>GSMSKWTYFGPDGENSWSKKYPSCGGLLQSPIDLHSDILQYDASLTPLEFQGYNLSANKQFLLTNNGHSVKLNLPSDMHIQGLQSRYSATQLHLHWGNPNDPHGSEHTVSGQHFAAELHIVHYNSDLYPDASTASNKSEGLAVLAVLIEMGSFNPSYDKIFSHLQHVKYKGQEAFVPGFNIEELLPERTAEYYRYRGSLTTPPCNPTVLWTVFRNPVQISQEQLLALETALYCTHMDDPSPREMINNFRQVQKFDERLVYTSFSQ[4x]

The role of carbonic anhydrase isozyme IX (CAIX) in tumor cell survival, proliferation, migration, pH regulation, and cell-signaling pathways made this enzyme a promising therapeutic target in oncology. , Tumor cells primarily express two membrane-associated carbonic anhydrases, CAIX and CAXII. These isozymes belong to a family of zinc metalloenzymes that catalyze the reversible hydration of CO2 to form HCO3 – and H+. Although the active site is characterized by conserved amino acids between 12 isozymes, the amino acids further away from the zinc ion provide some variability. Crystal structures of CAIX and CAXII with five compounds by using soaking or cocrystallization were determined to confirm the binding mode of the ligands and reveal insights that govern enhanced affinity.

Four ligands in complexes with CAXII are of similar structures, contain a cyclooctylamine group at the 3-position and (3-hydroxypropyl)­sulfonyl tail at the 4-position, but vary in substituents at the 5-position: compound 9 has a (4-hydroxybutyl)­amino moiety, compound 10 - piperidinyl, compound 13 - methoxy, and compound 14 - ethoxy. The introduction of methoxy (compound 13) and ethoxy (compound 14) groups at the 5-position of fluorinated benzenesulfonamide 5c resulted in the most strongly binding compounds for CAIX, with the K d,obs reaching 4.5 pM at pH 7.0. Interestingly, cancer-related CAXII also interacts strongly with 13 and 14, exhibiting 0.05 nM and 0.11 nM binding affinities, respectively. The tight binding of 13 to CAIX was confirmed by the ITC experiment, the slope of the integrated binding curve at pH 7.0 was extremely steep not allowing accurate determination of K d, however at pH 10 we obtained quite reasonable ITC binding isotherm with K d,obs around 26 nM. Complexes of CAXII-13 and CAXII-14 each have four subunits in both duplicate structures, and the ligands adopt nearly identical conformations across all eight subunits. First, the meta cyclooctylamino group is positioned in a hydrophobic region of the active site, making the main contacts with A129-S130 (main chain), V119, S133, and side chains of L197 and L139. In the structure containing compound 13 with a meta-methoxy group, a water molecule is consistently found between the ligand and protein, forming hydrogen bonds with Y6 and H67, but without a water-mediated hydrogen bond. The hydroxyl tail is oriented against the backbone of P200–P201, forming a hydrogen bond with the main chain oxygen of P200 in most subunits. Interestingly, despite the bulkiness of synthesized di-meta-substituted compounds 10, 13, and 14, especially the first one compound 10, which possesses large piperidinyl and cyclooctylamino groups, ligands acquire quite similar binding poses in the soaked and cocrystallized complexes with CAXII.7-({3-ethyl-5-[(methylamino)methyl]phenoxy}methyl)quinolin-2-amine | C20 H23 N3 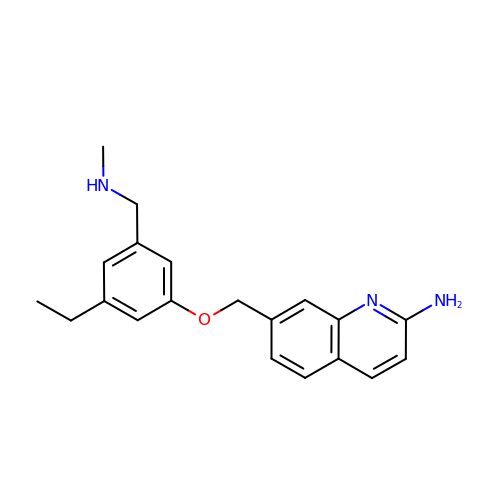O | OCTNSHZDWVJCQD-UHFFFAOYSA-N> DYGHSSPKPKLVRP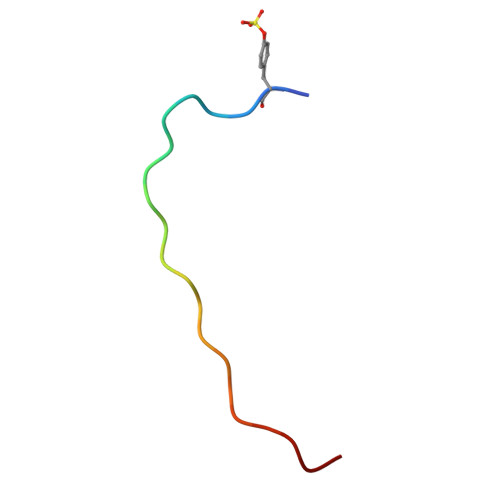PFKLIPN>AVSKVYARSVYDSRGNPTVEVELTTEKGVFRSIVPSGASTGVHEALEMRDGDKSKWMGKGVLHAVKNVNDVIAPAFVKANIDVKDQKAVDDFLISLDGTANKSKLGANAILGVSLAASRAAAAEKNVPLYKHLADLSKSKTSPYVLPVPFLNVLNGGSHAGGALALQEFMIAPTGAKTFAEALRIGSEVYHNLKSLTKKRYGASAGNVGDQGGVAPNIQTAEEALDLIVDAIKAAGHDGKVKIGLDCASSEFFKDGKYDLDFKNPNSDKSKWLTGPQ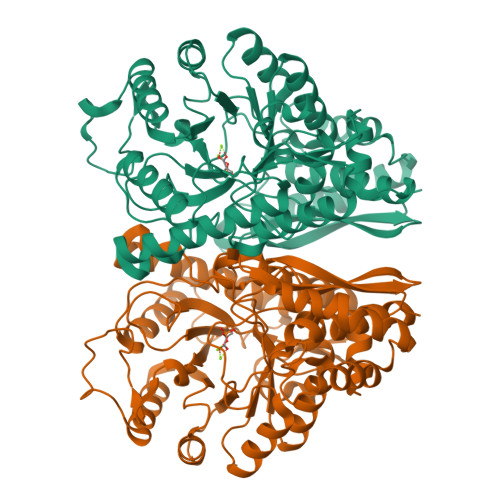LADLYHSLMKRYPIVSIEDPFAEDDWEAWSHFFKTAGIQIVADDLTVTNPKRIATAIEKKAADALLLKVNQIGTLSESIKAAQDSFAAGWGVMVSHRSGETEDTFIADLVVGLRTGQIKTGAPARSERLAKLNQLLRIEEELGDNAVFAGENFHHGDKL[2x]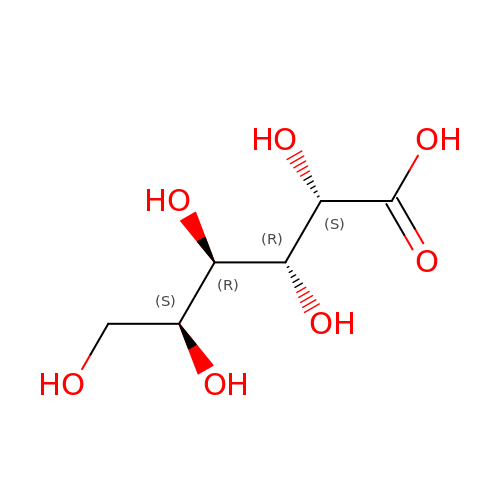L-galactonic acid | C6 H12 O7 | RGHNJXZEOKUKBD-RSJOWCBRSA-N> ACGCAGCCTGTACGGACATCAGATGCTGAGT;> CCGTACA;> GTACT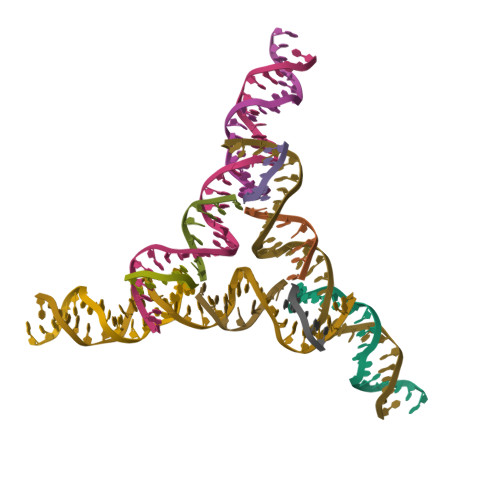CAGCATCTGATGT;> GGCTGC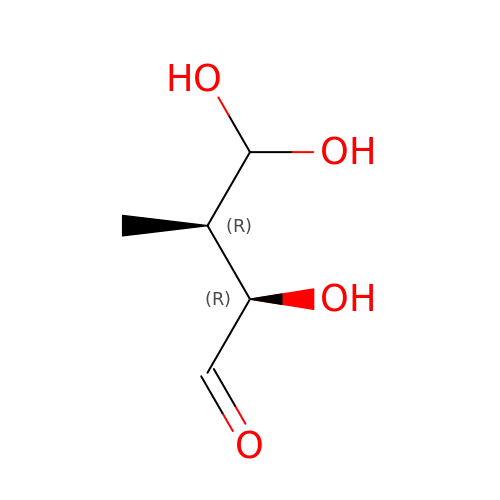(2R,3R)-2,4,4-trihydroxy-3-methylbutanal | C5 H10 O4 | NTSABUYTFOFFJR-DMTCNVIQSA-N>[2x]TSLYEIQM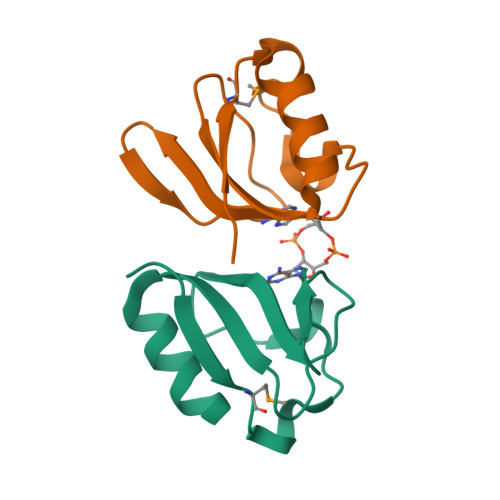LNYKYENIQLRNFPFGGDIIFVRIIRNNESIVPHGDTQLRYGDRLIVTGAKEYVDELKQELEFYF> MSNAEASRVYEIIVESVVNEVREDFENAGIDEQTLQ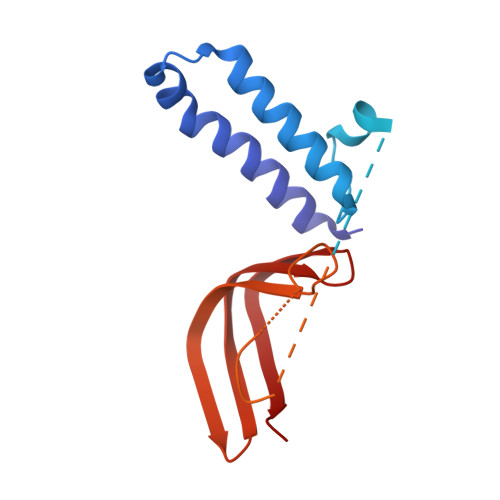DLKNIWQKKLTETKVTTFSWDNQFNEGNINGVQNDLNFNLATPGVNSSEFNIKEENTGNEGLILPNINSNNNIPHSGETNINTNTVEATNNSGATLNTNTSGNTNADVTSQPKIEVKPEIELTINNANITTVENIDDESEKKDDEEKEEDVEKTRKEKEQIEQVKLQAKKEKRSALLDTDEVGSELDDSDDDYLISEGEEDGPDENLMLCLYDKVTRTKARWKCSLKDGVVTINRNDYTFQKAQVEAEWV> MTDNLTTTHGGSTTLELLAQYNDHRSKKDKSIEHIEKGTCSGKERNPSYDEIFTENIKLKLQVQEYETEIESLEKVIDMLQKNREASLEVVLEQVQND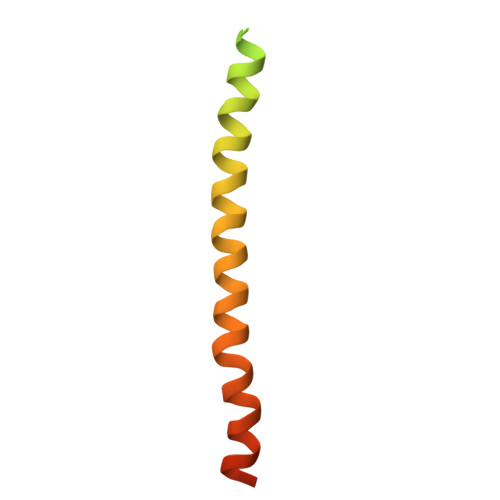S pirtobrutinib | C22 H21 F4 N5 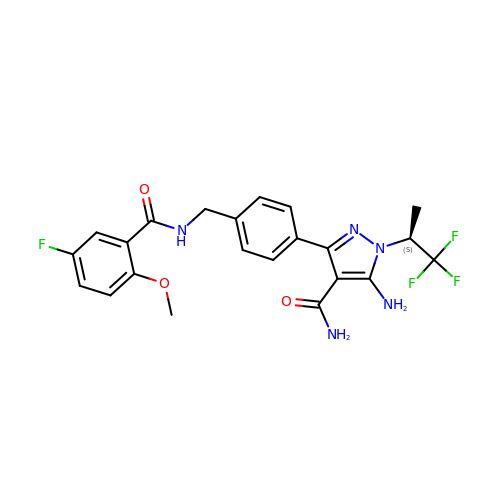O3 | FWZAWAUZXYCBKZ-NSHDSACASA-N>[2x]GHMSPNYDKWEMERTDITMKHKLGGGQYGEVYEGVWKKYSLTVAVKTLKEDTMEVEEFLKEAAVMKEIKHPNLVQLLGVCTREPPFYIITEFMTYGNLLDYLRECNRQEVNAVVLLYMATQISSAMEYLEKKNFIHRDLAARNCLVGENHLVKVADFGLSRLMTGDTYTAPAGAKFPIKWTAPESLAYNKFSIKSDVWAFGVLLWEIATYGMSPYPGIDLSQVYELLEKDYRMERPEGCPEKVYELMRACWQWNPSDRPSFAEIHQAFETMFQESSISDEVEKELGK;>[2x]AEEEIFGEFEAKK

BCR–Abl is a constitutively activated form of the nonreceptor tyrosine kinase c-Abl. The improper activation of the Abl tyrosine kinase results in chronic myeloid leukemia (CML). The recognition of an inactive conformation of Abl, in which a catalytically important Asp-Phe-Gly (DFG) motif is flipped by approximately 180° with respect to the active conformation, underlies the specificity of the cancer drug imatinib, which is used to treat CML. Our results suggest that interconversion between distinctly different inactive conformations is a characteristic feature of the Abl kinase domain.

The other structures include active and various inactive conformations that suggest how the kinase domain might convert between the αC-Glu In and αC-Glu Out conformations. (C) Active Abl (molecule C, structure 2). (D) In cells the active conformation of Abl undergoes rapid autophosphorylation that is expected to trap the protein in the active conformation (indicated as C*).> HHHHHHMDDSRSVNSVLLFTILNPIYSITTDVLYTICNPCGPVQRIVIFRKNGVQAMVEFDSVQSAQRAKASLNGADIYSGCCTLKIE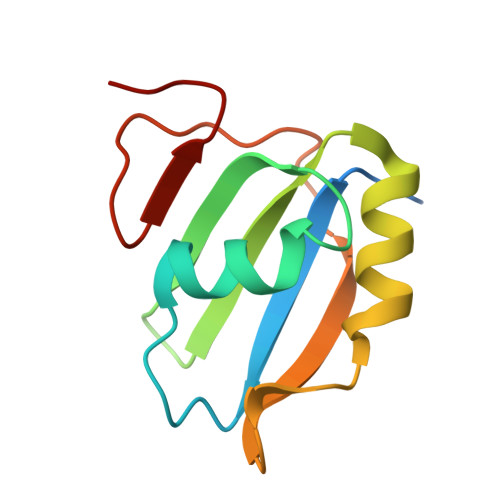YAKPTRLNVFKNDQDTWDYTNPN> GSLLDEIMAQTRCAPSEEGYDIAKKGVAAFIENLMGSQHSAEPVNKSLVDQMLVELDKKISAQMDEILHNSQFQAMESAWRGLKLFVDRTDFRENNKVEILHVTKDELLEDFEFAPETAQSGLYKHVYSAGYGQFGGEPVGAIIGNYAFTPSTPDMKLLQYMGALGAMAHAPFISSVGPEFFGIDSFEELPNIKDLKSTFESPKYTKWRSLRESEDARYLGLTAPRFLLRVPYDPIENPVKSFNYAENVSASHEHYLWGNTAFAFATRLTDSFAKYRWCPNIIGPQSGGAVEDLPVHVFESMGALQSKIPTEVLITDRKEFELAEEGFIALTMRKGSDNAAFFSANSI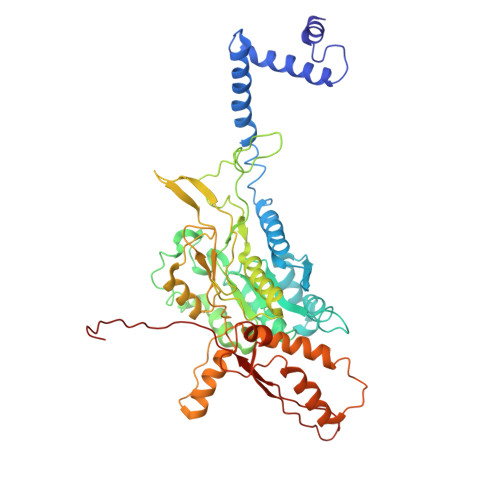QKPKVFPNTKEGKEAETNYKLGTQLPYMMIINRLAHYVKVLQREQIGAWKERQDLERELNSWIKQYVADQENPPADVRSRRPLRAARIEVMDVEGNPGWYQVSLSVRPHFKYMGANFELSLVGRL> AQPDIKFASKEYGVTIGESRIIYPLDAAGVMVSVKNTQDAPVLIQSRIYDENKEKESEDPFVVTPPLFRLDAKQQNSLRIAQAGGVFPRDKESLKWLCVKGIPPK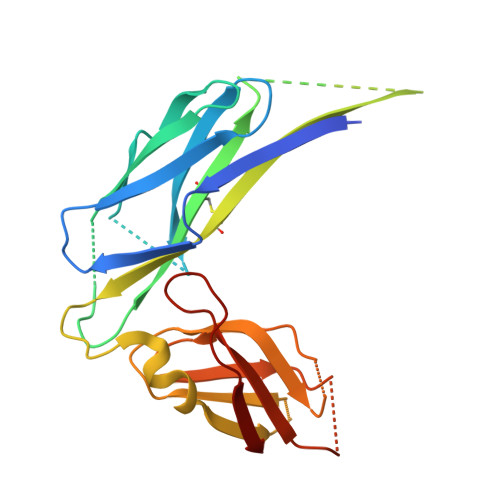DEDIWVDDATNKQKFNPDKDVGVFVQFAINNCIKLLVRPNELKGTPIQFAENLSWKVDGGKLIAENPSPFYMNIGELTFGGKSIPSHYIPPKSTWAFDLPKGLAGARNVSWRIINDQGGLDRLYSKNVTL>[4x]SMTLYSDQELAYLQQGEEAMQKALGILSNQEGWKKESQQDNGDKVMS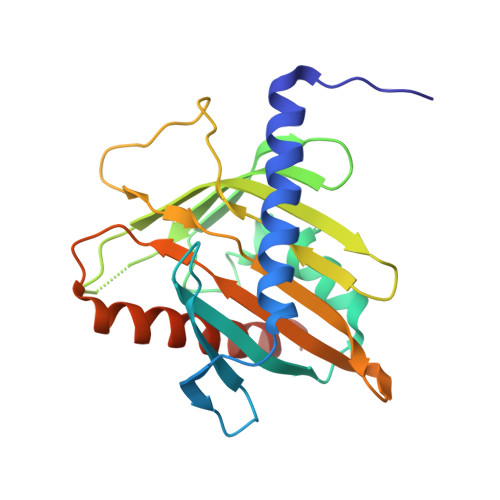KVVPDVGKVFRLEVVVDQPMERLYEELVERMEAMGEWNPNVKEIKVLQKIGKDTFITHELAAEAAGNLVGPRDFVSVRCAKRRGSTCVLAGMATDFGNMPEQKGVIRAEHGPTCMVLHPLAGSPSKTKLTWLLSIDLKGWLPKSIINQVLSQTQVDFANHLRKRLESHPASEAR>[2x]MLNSFKLSLQYILPKLWLTRLAGWGASKRAGWLTKLVIDLFVKYYKVDMKEAQKPDTASYRTFNEFFVRPLRDEVRPIDTDPNVLVMPADGVISQLGKI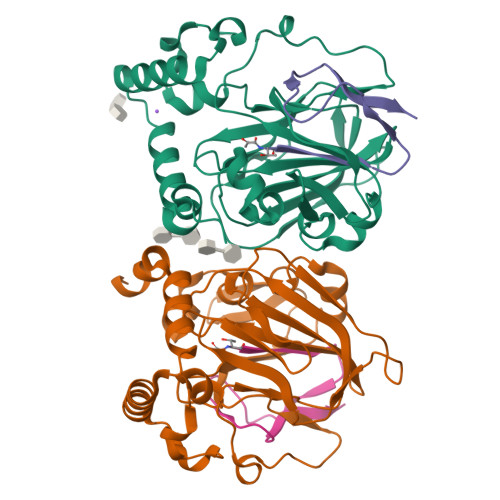EEDKILQAKGHNYSLEALLAGNYLMADLFRNGTFVTTYLSPRDYHRVHMPCNGILREMIYVPGDLFSVNHLTAQNVPNLFARNERVICLFDTEFGPMAQILVGATIVGSIETVWAGTITPPREGIIKRWTWPAGENDGSVALLKGQEMGRFKLG;>[2x]XTVINLFAPGKVNLVEQLESLSVTKIGQPLAVSTGHHHHHHG> EAASSSDADGKEVGSSGEGNRATGGKWRRPSLAQQRARRAQLPPAFD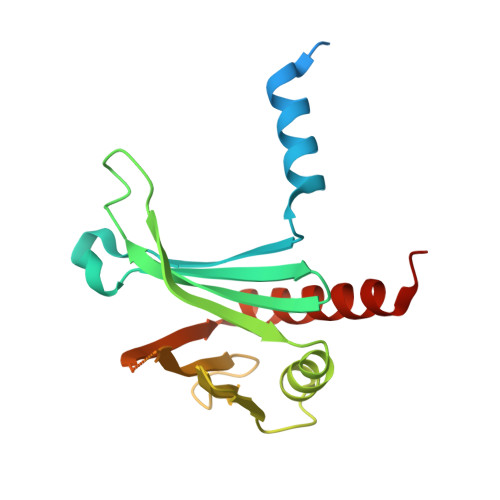VVHWNDEDISRGHLLRVLHRDTFVVLDYHRQARMLTEEGNKAERVVSVMLPAVYTARFLAVLEGRSEKVEVHSRYTNATFTPNPAAPYTFTLKCTSTRPAQQKQQVAGEEGDETFEWTVEFDVAESLMLQRFLTQALHYNTGFARTSV> SRYVKVYRKVMNLQRRKTPLPWTPTFLEFSKEPSVPFPVREKLQPAPIDLSYYLNMEVGDLVEVLHGPDCGRQGVVLSISKKRNTVVV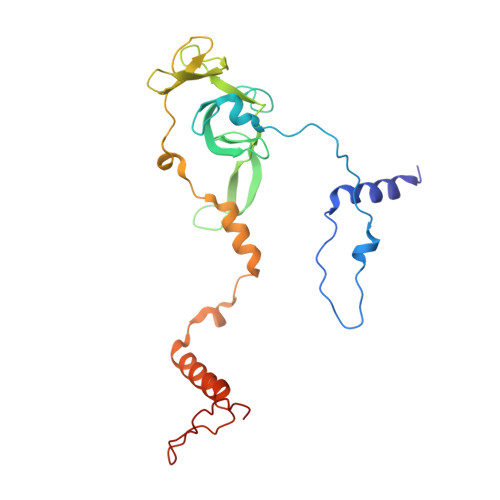DGCNMKKSFWNPGVGASLITQEMPIHITNVALLDPVVKRPTRVKRRFMMNGECVRISKLSGSAMPEPVSTSALRQPNLYQEYLRQKALGPPLKASYARPDPLHLKILQRLARHISWGQGSPLPTAENPRVNSPEPMALRR> MGIQGLAKLIADVAPSAIRENDIKSYFGRKVAIDASMSIYQFLIAVRQGGDVLQNEEGETTSHLMGMFYRTIRMMENGIKPVYVFDGKPPQLKSGELAKRSERRAEAEKQLQQAQAAGAEQEVEKFTKRLVKVTKQHNDECKHLLSLMGIPYLDAPSEAEASCAALVKAGKVYAAATEDMACLTFGSPVLMRHLTASEAKKLPIQEFHLSRILQELGLNQEQFVDLCILLGSDYCESIRGIGPKRAVDLIQKHKSIEEIVRRLDPNKY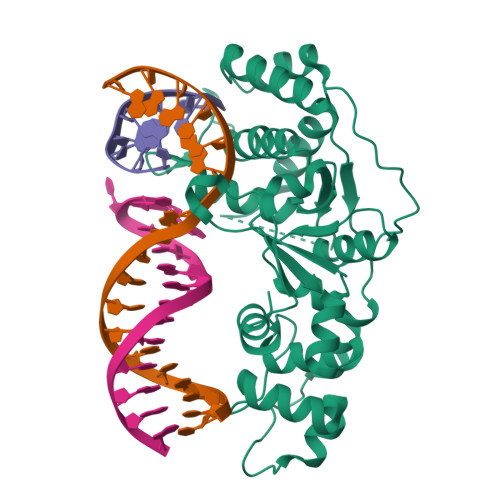PVPENWLHKEAHQLFLEPEVLDPESVELKWSEPNEEELIKFMCGEKQFSEERIRSGVKRLSKSRQ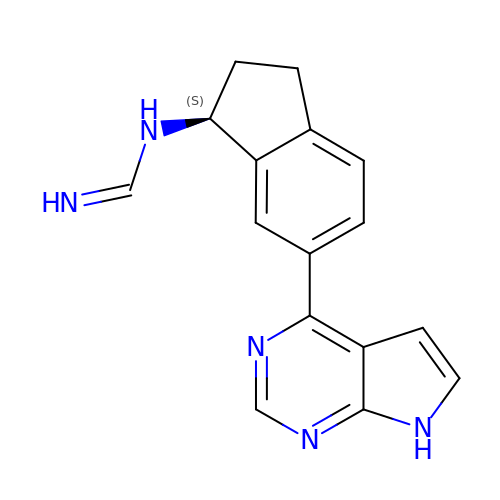N-[(1S)-6-(7H-pyrrolo[2,3-d]pyrimidin-4-yl)-2,3-dihydro-1H-inden-1-yl]imidoformamide | C16 H15 N5 | QXEVLNXNYUXLSG-AWEZNQCLSA-N>DYKDDDDKLHSQANLMRLKSDLFNRSPMYPGPTKDDPLTVTLGFTLQDIVKADSSTNEVDLVYYEQQRWKLNSLMWDPNEYGNITDFRTSAADIWTPDITAYSSTRPVQVLSPQIAVVTHDGSVMFIPAQRLSFMCDPTGVDSEEGATCAVKFGSWVYSGFEIDLKTDTDQVDLSSYYASSKYEILSATQTRQVQHYSCCPEPYID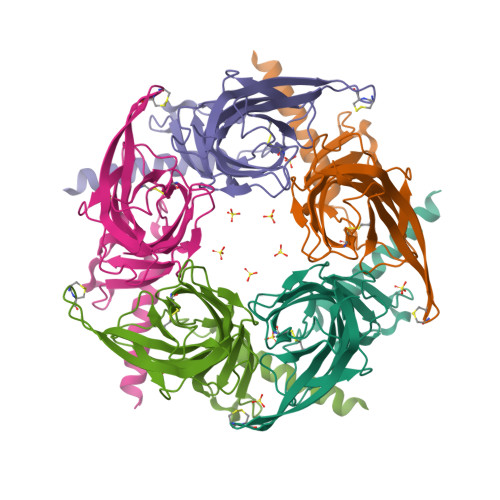VNLVVKFRERR[10x]>VGRALPDVRDGLKPVHRRVLYAMNVLGNDWNKAYKKSARVVGDVIGKYHPHGDSAVYDTIVRMAQPFSLRYMLVDGQGNFGSIDGDSAAAMRYTEIRLAKIAHELMADLEKETVDFVDNYDGTEKIPDVMPTKIPNLLVNGSSGIAVGMATNIPPHNLTEVINGCLAYIDDEDISIEGLMEHIPGPDFPTAAIINGRRGIEEAYRTGRGKVYIRARAEVEVDAKTGRETIIVHEIPYQVNKARLIEKIAELVKEKRVEGISALRDESDKDGMRIVIEVKRDAVGEVVLNNLYSQTQLQVSFGINMVALHHGQPKIMNLKDIIAAFVRHRREVVTRRTIFELRKARDRAHILEALAVALANIDPIIELIRHAPTPAEAKTALVANPWQLGNVAAMLERAGDDAARPEWLEPEFGVRDGLYYLTEQQAQAILDLRLQKLTGLEHEKLLDEYKELLDQIAELLRILGSADRLMEVIREELELVREQFGDKRRTEIT[2x]

DNA gyrase is the only type II topoisomerase capable of catalyzing DNA supercoiling, in a reaction driven by ATP hydrolysis. DNA gyrase consists of two subunits, GyrA and GyrB (97 kDa and 90 kDa, respectively, in Escherichia coli), forming an A2B2 complex in the active enzyme. The N-terminal domain of GyrB is the site of ATP hydrolysis, while DNA cleavage and strand passage occur at the interface between the C-terminal domain of GyrB and the N-terminal domain of GyrA. A new GyrA NTD fragment was constructed with a view of obtaining a crystal structure of SD8 bound to GyrA in an alternative conformation that would be representative of the situation at lower ligand concentrations. This smaller 55-kDa NTD fragment of GyrA (GyrA55), comprising residues 30–522 of the 875-amino-acid wild-type sequence (compared with residues 2–522 for GyrA59), crucially lacks residues spanning Leu17 to Asp23 that have been identified as providing 10 of the 12 protein–protein hydrogen bonds responsible for stabilizing the tetramer at the dimer–dimer interface in the crystal structure of the GyrA59–SD8 complex.

The 2.05-Å-resolution GyrA55–SD8 complex structure contains two GyrA55 monomers in the ASU, although they do not form the biologically relevant homodimer. Instead, two distinct homodimers can be generated from these monomers by the addition of crystallographic symmetry-related monomers. One of the resultant homodimers binds two crystallographically equivalent SD8 molecules in a novel conformation. The conformation of the SD8 in GyrA55–SD8 is significantly different to that observed in the previous study, principally because it is bound entirely within one GyrA55 homodimer. The polyketide moiety has shifted to a position where it spans the interface between the two GyrA monomers, with SD8 forming hydrogen-bonding interactions with residues from each monomer, specifically as follows: direct hydrogen-bonding interactions with His80, Gly81, and Met120 (from the adjacent monomer) and indirect hydrogen-bonding interactions (via water molecules) with Pro79 and Asp87 (from the adjacent monomer). The aminocoumarin moiety is bound to the protein through hydrogen-bonding interactions with Lys42, His45, Arg91, and Ser172 and hydrophobic contacts with Val44. In order to accommodate SD8 in this new binding configuration, a single cis bond is required in the tetraene linker adjacent to the ester linkage with the olivose and is fully consistent with the observed electron density. The only significant change is that the N-terminal end of α-helix 3 partially unwinds (it becomes two residues shorter), allowing the protein main chain in this region to move in order to accommodate the polyketide moiety of one SD8 molecule and, in so doing, projects the side chain of Asp87 toward the symmetry-related SD8 molecule, such that it hydrogen bonds, via a water molecule, to the ester group connecting the tetraene linker to the olivose sugar.> MAAGVPCALVTSCSSVFSGDQLVQHILGTEDLIVEVTSNDAVRFYPWTIDNKYYSADINLCVVPNKFLVTAEIAESVQAFVVYFDSTQKSGLDSVSSWLPLAKAWLPEVMILVCDRVSEDGINRQKAQEWCIKHGFELVELSPEELPEEDDDFPESTGVKRIVQALNANVWSNVVMK;> MIHFILLFSRQGKLRLQKWYITLPDKERKKITREIVQIILSRGHRTSSFVDWKELKLVYKRYASLYFCCAIENQDNELLTLEIVHRYVELLDKYFGNVCELDIIFNFEKAYFILDEFIIGGEIQETSKKIAVKAIEDSDMLQEVSTVSQT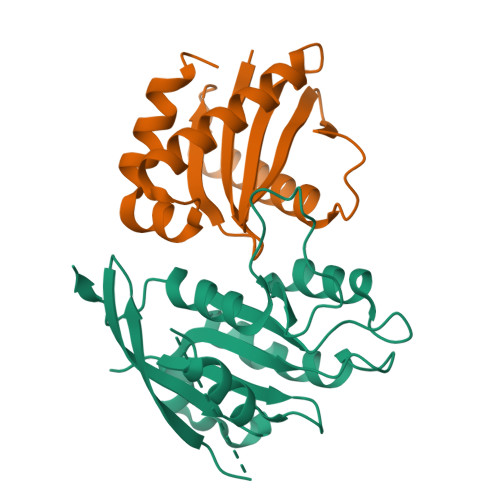MGER5-amino-2,4,6-tribromobenzene-1,3-dicarboxylic acid | C8 H4 Br3 N O4 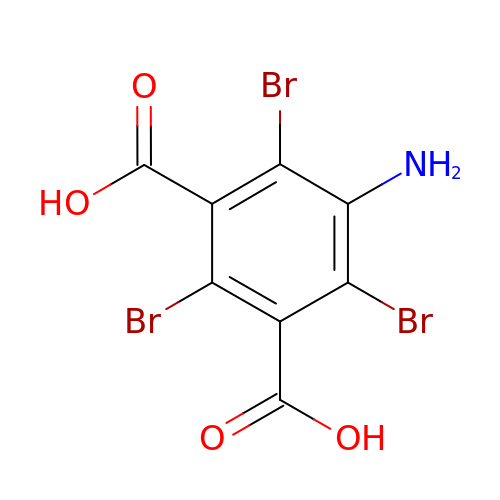| KGKQFJKPOZCZLD-UHFFFAOYSA-N>GPGHMAERTWIFSGAELKQAIEGKLAPDVSDPEMRRLVSVAKSSAYIAGVADLTSGSDWCGAGAVAPHELTDRIY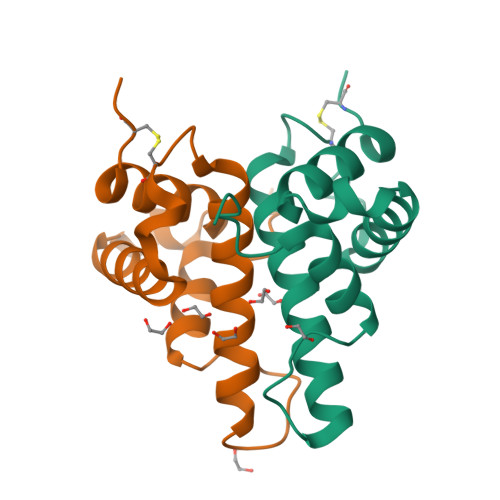TYLGDMPAEKLDEQAATLVREALKVSFPCEQKSN[2x]>[4x]SSEDKITVHFINRDGETLTTKGKIGDSLLDVVVQNNLDIDGFGACEGTLACSTCHLIFEQHIFEKLEAITDEENDMLDLAYGLTDR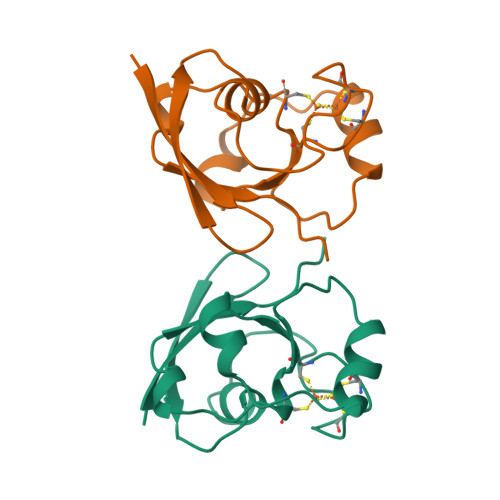SRLGCQICLTKAMDNMTVRVPDAVSDARESIDMGMNSSKIE>[2x]MLLARMNPQVQPENNGADTGPEQPLRARKTAELLVVKERNGVQCLLAPRDGDAQPRETWGKKIDFLLSVVGFAVDLANVWRFPYLCYKNGGGAFLIPYTLFLIIAGMPLFYMELALGQYNREGA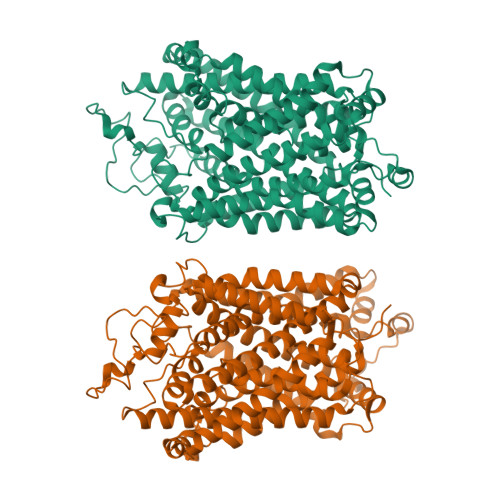ATVWKICPFFKGVGYAVILIALYVGFYYNVIIAWSLYYLFSSFTLNLPWTDCGHTWNSPNCTDPKLLNGSVLGNHTKYSKYKFTPAAEFYERGVLHLHESSGIHDIGLPQWQLLLCLMVVVIVLYFSLWKGVKTSGKVVWITATLPYFVLFVLLVHGVTLPGASNGINAYLHIDFYRLKEATVWIDAATQIFFSLGAGFGVLIAFASYNKFDNNCYRDALLTSSINCITSFVSGFAIFSILGYMAHEHKVNIEDVATEGAGLVFILYPEAISTLSGSTFWAVVFFVMLLALGLDSSMGGMEAVITGLADDFQVLKRHRKLFTFGVTFSTFLLALFCITKGGIYVLTLLDTFAAGTSILFAVLMEAIGVSWFYGVDRFSNDIQQMMGFRPGLYWRLCWKFVSPAFLLFVVVVSIINFKPLTYDDYIFPPWANWVGWGIALSSMVLVPIYVIYKFLSTQGSLWERLAYGITPENEHHLVAQRDIRQFQLQHWLAI>MDNSIHSTDGPDSVIPNSNPKKTVRQRVRLLARHLTTREGLIGDYDYGFLFRPELPFMKKDPRAPPFFGLNEKIPVLLAFILGLQHALAMLAGVVTPPLIISSSLSLPSDLQQYLVSTSLIVCGLLSMVQITRFHIYKTPYYIGSGVLSVMGVSFSIISVASGAFNQMYSNGFCQLDEAGNRLPCPEAYGALIGTSACCALVEILLAFVPPKVIQKIFPPIVTGPTVMLIGISLIGTGFKDWAGGSACMDDGMLCPSATAPRPLPWGSPEFIGLGFLVFVSIILCE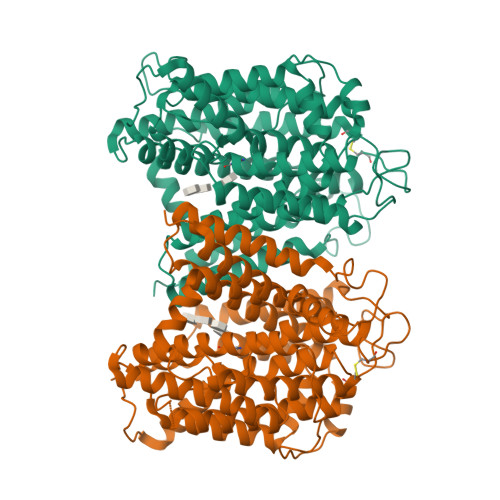RFGAPIMKSCSVVIGLLVGCIVAAACGYFSHADIDAAPAASFIWVKTFPLSVYGPMVLPIIAVFIICACECIGDVTATCDVSRLEVRGGTFESRIQGAVLADGINSVVAALATMTPMTTFAQNNVVIALTRCANRWAGYCCCLILIVAGIFAKFAAAIVAIPNSVMGGMKTFLFASVVISGQAIVAKAPFTRRNRFILTASMALGYGATLVPTWFGNVFPQTENRDLEGFENAIELVLETGFAVTAFVAMLLNAIMPAEVEEIGAVTPMPVSAHDNRDGEAEYQSKQA[2x]>SKMSDVKCTSVVLLSVLQQLRVESSSKLWAQCVQLHNDILLAKDTTEAFEKMVSLLSVLLSMQGAVDINKL[2x];>SEDKRAKVTSAMQTMLFTMLRKLDNDALNNIINNARDGCVPLNIIPLTTAAKLMVVIPDYNTYKNTCDGTTFTYASALWEIQQVVDADSKIVQLSEISMDN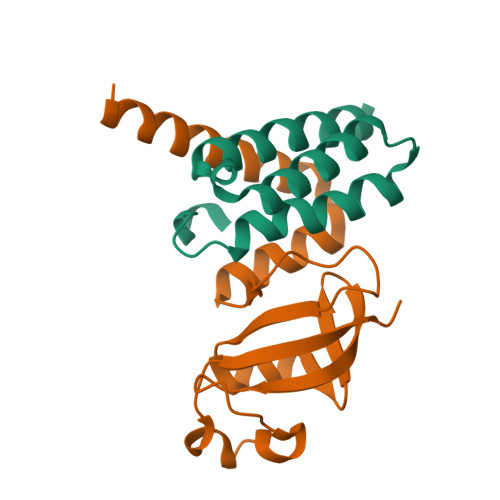SPNLAWPLIVTALRAN[2x]> MGSDKIHHHHHHENLYFQGMRYLSKDILEEVITQRPSDSYKSNFGRVVLIGGNRQYGGAIIMSTEACINSGAGLTTVITDVKNHGPLHARC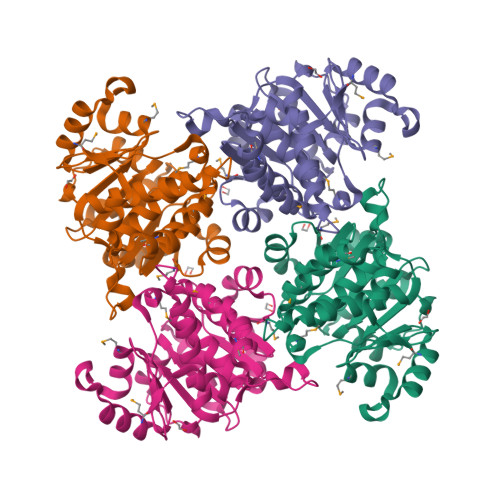PEAMVVGFEETVLLTNVVEQADVILIGPGLGLDATAQQILKMVLAQHQKQQWLIIDGSAITLFSQGNFSLTYPEKVVFTPHQMEWQRLSHLPIEQQTLANNQRQQAKLGSTIVLKSHRTTIFHAGEPFQNTGGNPGMATGGTGDTLAGIIAGFLAQFKPTIETIAGAVYLHSLIGDDLAKTDYVVLPTKISQALPTYMKKYAQPHTAPDSELLEQKRSR> 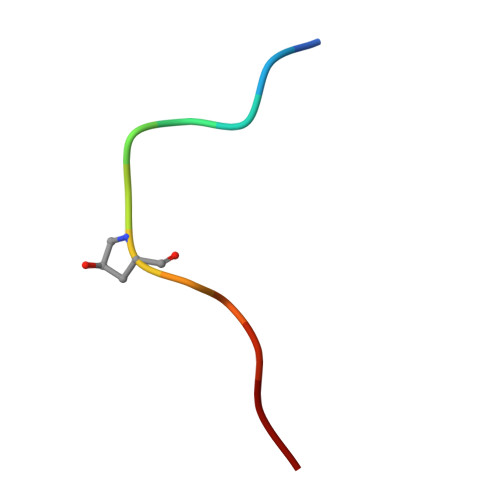PIPPSAPSKRHN>[2x]MELYRDPSQPIEVRVRDLLSRMTLEEKVAQLGSVWGYELIDERGKFSREKAKELLKNGIGQITRPGGSTNLEPQEAAELVNEIQRFLVEETRLGIPAMIHEECLTGYMGLGGTNFPQAIAMASTWDPDLIEKMTTAVREDMRKIGAHQGLAPVLDVARDPRWGRTEETFGESPYLVARMGVSYVKGLQGEDIKKGVVATVKHFAGYSASEGGKNWAPTNIPEREFKEVFLFPFEAAVKEANVLSVMNSYSEIDGVPCAANRKLLTDILRKDWGFEGIVVSDYFAVKVLEDYHRIARDKSEAARLALEAGIDVELPKTECYQYLKDLVEKGIISEALIDEAVTRVLRLKFMLGLFENPYVEVEKAKIESHRDIALEIARKSIILLKNDGILPLQKNKKVALIGPNAGEVRNLLGDYMYLAHIRALLDNIDDVFGNPQIPRENYERLKKSIEEHMKSIPSVLDAFKEEGIEFEYAKGCEVTGEDRSGFEEAIEIAKKSDVAIVV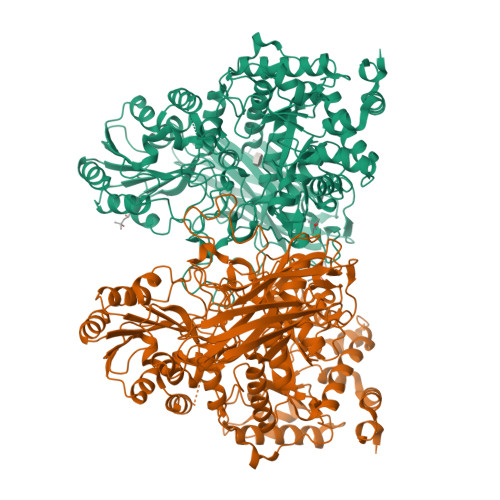VGDKSGLTLDCTTGESRDMANLKLPGVQEELVLEVAKTGKPVVLVLITGRPYSLKNVVDKVNAILQVWLPGEAGGRAIVDIIYGKVNPSGKLPISFPRSAGQIPVFHYVKPSGGRSHWHGDYVDESTKPLFPFGHGLSYTKFEYSNLRIEPKEVPPAGEVVIKVDVENIGDRDGDEVVQLYIGREFASVTRPVKELKGFKRVSLKAKEKKTVVFRLHMDVLAYYNRDMKLVVEPGEFKVMVGSSSEDIRLTGSFSVVGEKREVVGMRKFFTEACEEAAALEENLYFQGAHHHHHHHHHH>MSAKSRTIGIIGAPFSKGQPRGGVEEGPTVLRKAGLLEKLKEQECDVKDYGDLPFADIPNDSPFQIVKNPRSVGKASEQLAGKVAEVKKNGRISLVLGGDHSLAIGSISGHARVHPDLGVIWVDAHTDINTPLTTTSGNLHGQPVSFLLKELKGKIPDVPGFSWVTPCISAKDIVYIGLRDVDPGEHYILKTLGIKYFSMTEVDRLGIGKVMEETLSYLLGRKKRPIHLS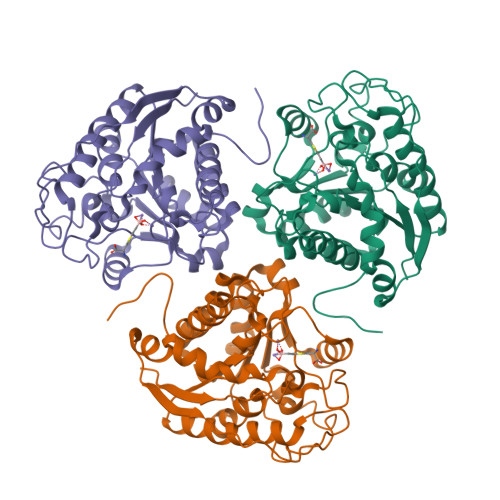FDVDGLDPSFTPATGTPVVGGLTYRQGLYITEEIYKTGLLSGLDIMEVNPSLGKTPEEVTRTVNTAVAITLACFGLAREGNHKPIDYLNPPK[2x]> MTTTERPDLAWLDEVTMTQLERNPYEVYERLRAEAPLAFVPVLGSYVASTAEVCREVATSPDFEAVITPAGGRTFGHPAIIGVNGDIHADLRSMVEPALQPAEVDRWIDDLVRPIARRYLERFENDGHAELVAQYCEPVSVRSLGDLLGLQEVDSDKLREWFAKLNRSVTNAAVDENGEFANPEGFAEGDQAKAEIRAVVDPLIDKWIEHPDDSAISHWLHDGMPPGQTRDREYIYPTIYVYLLGAMQEPGHGMASTLVGLFSRPEQLEEVVDDPTLIPRAIAEGLRWTSPIWSATARISTKPVTIAGVDLPAGTPVMLSYGSANHDTGKYEAPSQYDLHRPPLPHLAFGAGNHACAGIYFANHVMRIALEELFE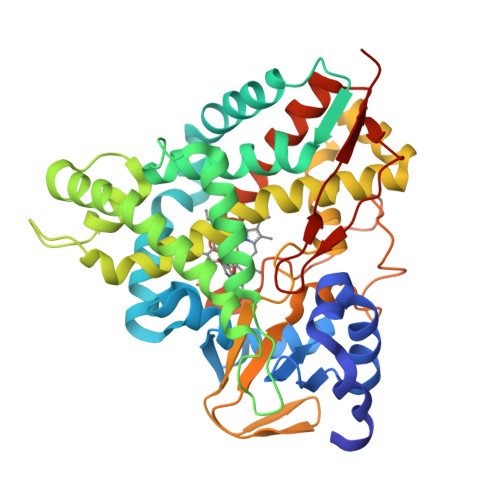AIPNLERDTREGVEFWGWGFRGPTSLHVTWEV1-((1R)-1-(HYDROXYMETHYL)-3-PHENYLPROPYL)-1H-IMIDAZOLE-4-CARBOXAMIDE | C14 H17 N3 O2 | 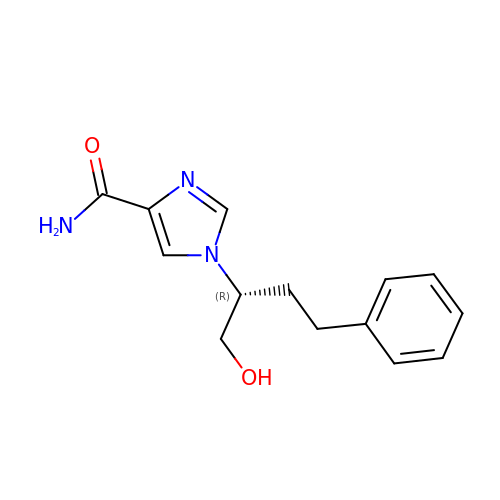ZUYUIKKHHBEVHL-GFCCVEGCSA-N>SPPQKVCLICGDEASGCHYGVLTCGSCKVFFKRAVEGQHNYLC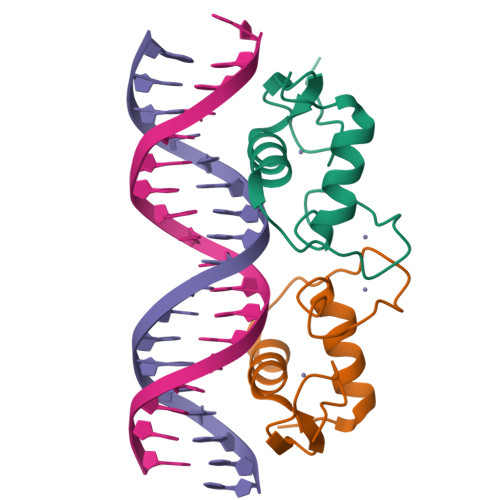AGRNDCIIDKIRRKNCPACRLRKCLQAGMTLGARKSKKL[4x]> LFIEWL

Here, we identify an evolutionarily conserved hexapeptide sequence as the major aggregation-prone region (APR) of gastrointestinal peptides of the glucagon family: xFxxWL. We determine nine polymorphic crystal structures of the APR segments of glucagon-like peptides 1 and 2, and exendin and its derivatives. We propose that the pH-dependent changes of the protonation states of glutamate/aspartate residues of APRs initiate switching between the amyloid and the folded, monomeric forms of the hormones. Our results highlight the dual role of short aggregation core motifs in reversible amyloid formation and receptor binding.

Two polymorphic crystal forms could be grown from solutions of APRex-4. In the case of polymorph A, side chains presented an unusually high degree of flexibility. Side chains of Phe2 and the partially disordered side chain of Trp5 assembled into an aromatic cluster near the solvent channel and chain termini. The hydrophobic core is formed by Leu1 and Leu6 while intrasheet H-bonds of Glu-Glu side chains stabilize the interface. The weak residual electron density around the side chains of Trp5 suggests that additional conformers of this side chain are also present in the otherwise close-packed crystals. Tryptophan of LFIEWL (polymorph A) adopts different conformational states, (opaque and transparent side chains) having multiple geometries of aromatic interactions. An aromatic cluster is formed in both polymorphs of APRex-4. However, the exact geometry of the cluster in polymorph A is ambiguous due to the elevated internal mobility of the Trp side chain. At pHs where Glu/Asp side chains become protonated, charge frustration ceases as side chains establish intersheet H-bonds. For example, protonated Glu forms H-bond either with the opposing Glu (S1 of polymorph A, S3 of Polymorph B in APRex-4 Fig. 6c), or with the indole rings of Trp(s) (S2 of Polymorph B Fig. 4e). In the presence of organic solvents, the exendin-like structures adopted more compact crystal forms, in which opposing side chains of the steric zippers interact with each other.> PLSVDSKTVNYFDIITIKHQDTDAFLHSHLARYPQRYEDGRISSA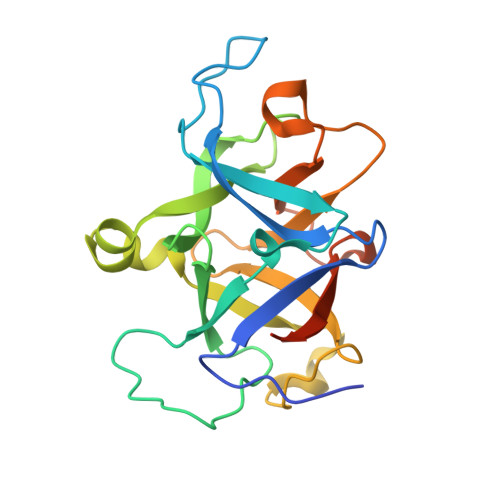GQQVTGYTHPDFNNQWEVLPPHGSDVGKGQAVLLNQHIRLRHVATDTYLLAHDVASPFYPTNEEITTVTLEEGDGELYPETLFAFQPLKKSDEGHVLKSKTVSFRLFHVDTSVALWTHNDELLPDWGFQQQEINGNKKVIDPSNNWVVDEIVNLDEVRKVYIPKVV> HENIDWGEPKD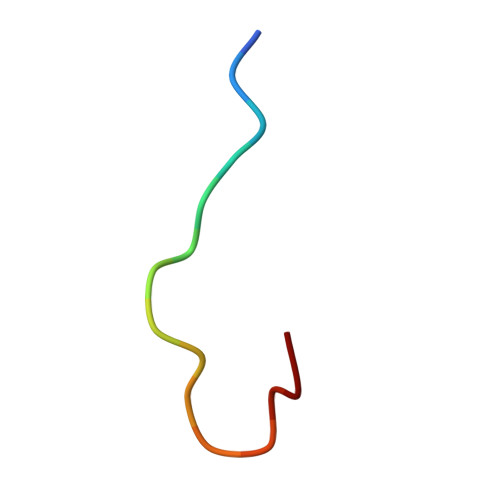KEVW>[4x]FETRFEKMDNLLRDPKSEVNSDCLLDGLDALVYDLDFPALRKNKNIDNFLSRYKDTINKIRDLRMKAEDYEVVKVIGRGAFGEVQLVRHKSTRKVYAMKLLSKFEMIKRSDSAFFWEERDIMAFANSPWVVQLFYAFQDDRYLYMVMEYMPGGDLVNLMSNYDVPEKWARFYTAEVVLALDAIHSMGFIHRDVKPDNMLLDKSGHLKLADFGTCMKMNKEGMVRCDTAVGTPDYISPEVLKSQGGDGYYGRECDWWSVGVFLYEMLVGDTPFYADSLVGTYSKIMNHKNSLTFPDDNDISKEAKNLICAFLTDREVRLGRNGVEEIKRHLFFKNDQWAWETLRDTVAPVVPDLSSDIDTSNFDDLEEDKGEEETFPIPKAFVGNQLPFVGFTYYSN

We apply this method to identify inhibitors of ROCK1 from almost one billion commercially available compounds. To facilitate further validation of the method and confirm the postulated binding modes, we obtained co-crystal structures of ROCK1 in complex with Compound 1, the most potent inhibitor identified in the virtual screening campaign, and with Compound 22, an inhibitor we considered structurally unique. The crystals contained four monomers of the ROCK1 kinase domain in the asymmetric unit, of which chains A, B, and C were relatively well defined, while the fourth copy of chain D was quite poorly ordered and not used in analyses. Focusing on the chain A example in each structure, the resulting electron density shows a clear binding mode for each ligand.

The pyrazole class was the most populous, with fifteen active molecules. Examination of their docked poses revealed that they contained a phenyl group distal to the hydrogen bonding N-N pair of the pyrazole. This phenyl-pyrazole moiety fills a similar volume to that of the purine group in a native ATP-bound kinase structure. In addition to the phenyl group, all actives contained a C- or N-linked amide group at the para position to the pyrazole, providing the connection to the hydrophobic P-loop group. The structures were solved and refined to a final resolution of 2.34 Å (Compound 1) and 2.74 Å (Compound 22). With the Compound 1 example, the pyrazole nitrogens that bind the hinge motif are 0.8 or 1.0 Å apart between the experimental structure and the docked model, while the alignment of the protein atom component of these hydrogen bonds show 0.4 or 0.6 Å separations. The mid-ligand phenyl linker ring has a distinct tilt in the experimental structure, but the overall ligand position remains co-located with the docked model. This is despite a large difference in the protein structures where our crystal structure model was built, interpreting density to indicate an inversion of the DFG motif (which also leads into a disordered activation loop) such that the inward location of the phenylalanine 217 sidechain creates a very different platform surface for the base of the ligand binding pocket. Since docking protocols generally do not account for such large conformational changes and protein dynamics, the consistency of the experimental and docked ligand poses in this example are all the more remarkable.9-(4-HYDROXY-3-(HYDROXYMETHYL)BUT-1-YL)GUANINE 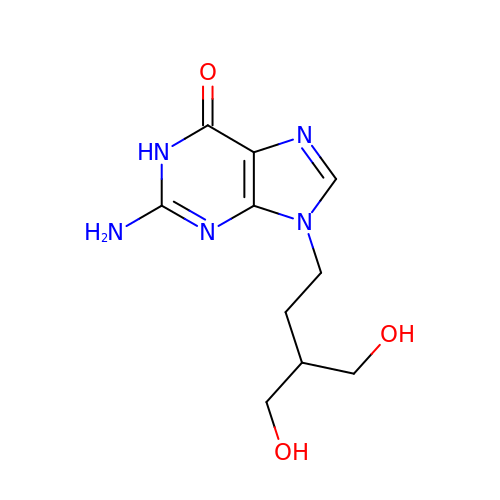| C10 H15 N5 O3 | JNTOCHDNEULJHD-UHFFFAOYSA-N>[2x]MHGAFSTNVVASKELQQPGSARSTRHLEIELPKEASYQEGDHLGVIPRNYEGIVNRVTARFGLDASQQIRLEAEEEKLAHLPLAKTVSVEELLQYVELQDPVTRTQLRAMAAKTVAPPHKVELE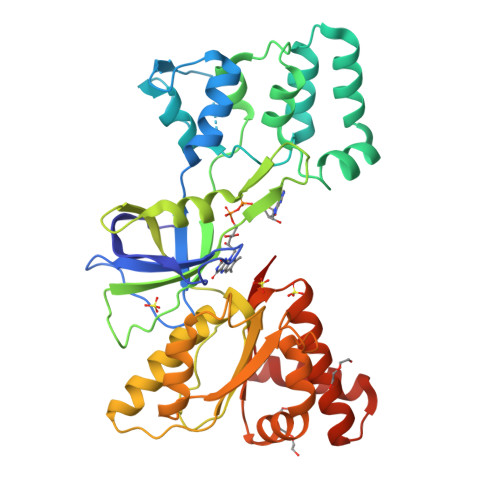ALLEKQAYKEQVLAKRLTMLELLEKYPACEMKFSEFIALLPSIRPRYYSISSSPRVDEKQASITVSVVSGEAWSGYGEYKGIASNYLAELQEGDTITCFISTPQSEFTLPKDPETPLIMVGPGTGVAPFRGFVQARKQLKEQGQSLGEAHLYFGCRSPHEDYLYQEELENAQSEGIITLHTAFSRMPNQPKTYVQHVMEQDGKKLIELLDQGAHFYICGDGSQMAPAVEATLMKSYADVHQVSEADARLWLQQLEEKGRYAKDVWAG> YSNCGENEYYNQTTGLCQECPPCGPGEEPYLSCGYGTKDEDYGCVPCPAEK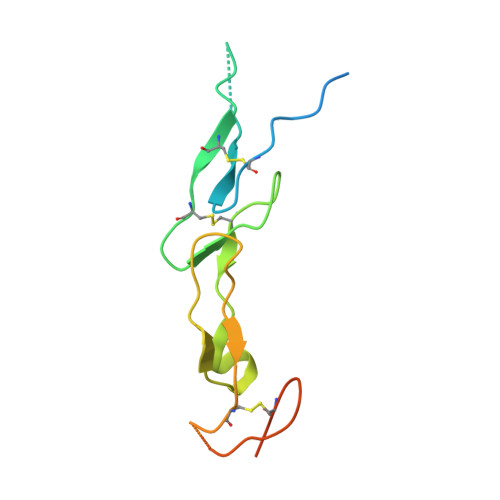FSKGGYQICRRHKDCEGFFRATVLTPGDMENDAECGPCLPGYYMLENRPRNIYGMVCYSCLLAPPNTKECVG>[4x]SGFVCNTCPEKWINF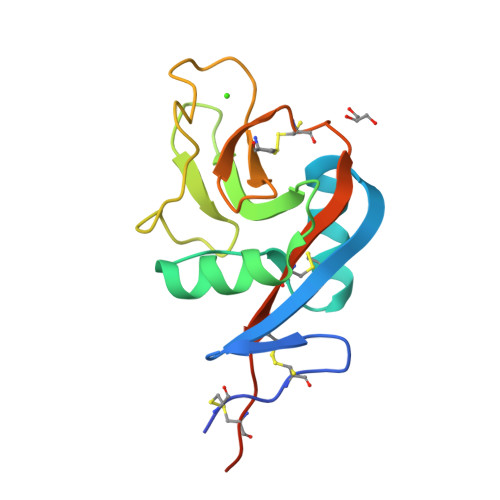QRKCYYFGKGTKQWVHARYACDDMEGQLVSIHSPEEQDFLTKHASHTGSWIGLRNLDLKGEFIWVDGSHVDYSNWAPGEPTSRSQGEDCVMMRGSGRWNDAFCDRKLGAWVCDRLATCTPPASEGSAE N-(4-methylphenyl)-1H-pyrazolo[3,4-d]pyrimidin-4-amine 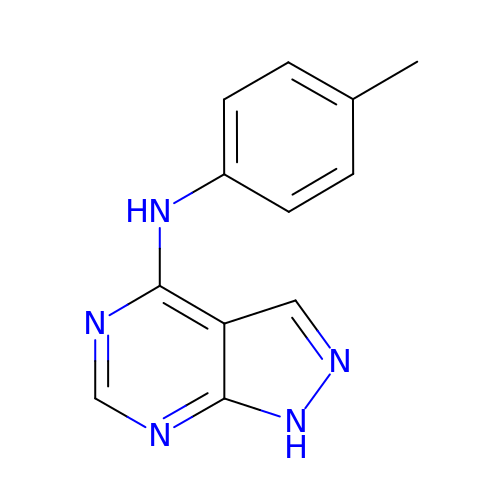| C12 H11 N5 | TZIUGCYEFCFJRQ-UHFFFAOYSA-N>GGSYSKSPSNKDAALLEAARANNMQEVSRLLSEGADVNAKHRLGWTALMVAAINRNNSVVQVLLAAGADPNLGDDFSSVYKTAKEQGIHSLEDGGQDGASRHITNQWTSALEFRRWLGLPAGVLITREDDFNNRLNNRASFKGCTALHYAVLADDYRTVKELLDGGANPLQRNEMGHTPLDYAREGEVMKLLRTSEAKYQEKQRKREAEERRRFPLEQRLKEHIIGQESAIATVGAAIRRKENGWYDEEHPLVFLFLGSSGIGKTELAKQTAKYMHKDAKKGFIRLDMSEFQERHEVAKFIGSPPGYVGHEEGGQLTKKLKQCPNAVVLFDEVDKAHPDVLTIMLQLFDEGRLTDGKGKTIDCKDAIFIMTSNVASDEIAQHALQLRQEALEMSRNRIAENLGDVQISDKITISKNFKENVIRPILKAHFRRDEFLGRINEIVYFLPFCHSELIQLVNKELNFWAKRAKQRHNITLLWDREVADVLVDGYNVHYGARSIKHEVERRVVNQLAAAYEQDLLPGGCT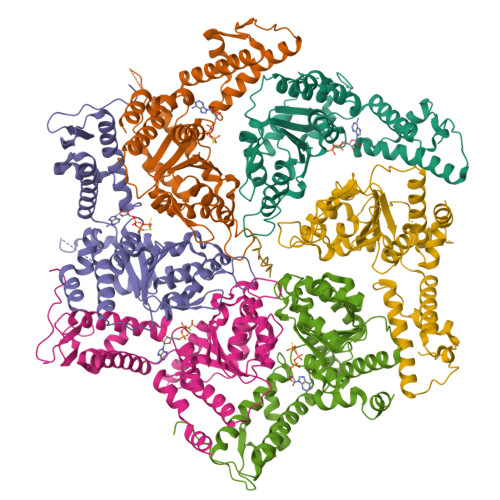LRITVEDSDKQLLKSPELPSPQAEKRLPKLRLEIIDKDSKTRRLDIRAPLHPEKVCNTI[6x];> XXXXXXXXXXXXXXARELEELNVPGEIVESLSSSEESITRINKKIEKFQSEEQQQTEDELQDKIHPFAQTQSLVYPFPGPIPNSLPQNIPPLTQTPVVVPPFLQPEVMGVSKVKGAMAPKHKEMPFPKYPVEPLTESQSLTLTDVENLHLPLPLLQSWMHQPHQPLPPTVMFPPQSVLSLSQSKVLPVPQKAVPYPQRDMPIQAFLLYQEPVLGPVRGPFPIIV> MAYPNDQQGKALPFFARFLSVSKEESSIKSPSPDHEIS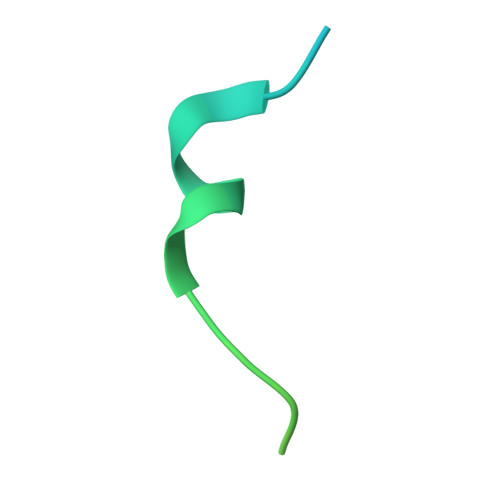TRKYPSDWEEW> GGYVAPKAVWLPAVKAKGLEISGTFTHRQGHIYMEMNFTNKALQHMTDFAIQFNKNSFGVIPSTPLAIHTPLMPNQSIDVSLPLNTLGPVMKMEPLNNLQVAVKNNIDVFYFSCLIPLNVLFVEDGKMERQVFLATWKDIPNENELQFQIKECHLNADTVSSKLQNNNVYTIAKRNVEGQDMLYQSLKLTNGIWILAELRIQPGNPNYTLSLKC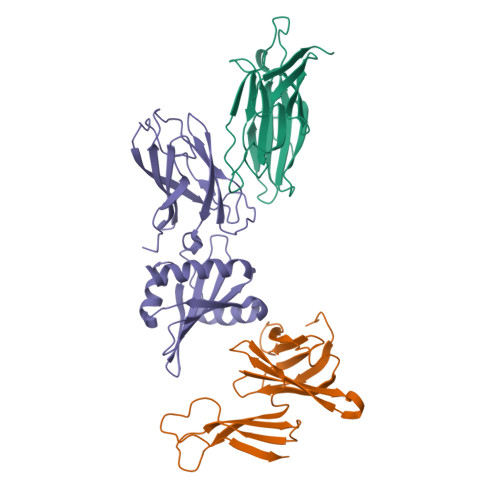RAPEVSQYIYQVYDSILKN;>[2x]MAQILPIRFQEHLQLQNLGINPANIGFSTLTMESDKFICIREKVGEQAQVVIIDMNDPSNPIRRPISADSAIMNPASKVIALKAGKTLQIFNIEMKSKMKAHTMTDDVTFWKWISLNTVALVTDNAVYHWSMEGESQPVKMFDRHSSLAGCQIINYRTDAKQKWLLLTGISAQQNRVVGAMQLYSVDRKVSQPIEGHAASFAQFKMEGNAEESTLFCFAVRGQAGGKLHIIEVGTPPTGNQPFPKKAVDVFFPPEAQNDFPVAMQISEKHDVVFLITKYGYIHLYDLETGTCIYMNRIS>[12x]MPIVVTQAHIDRVGIAADLLDASPVSLQVLGRPTAINTV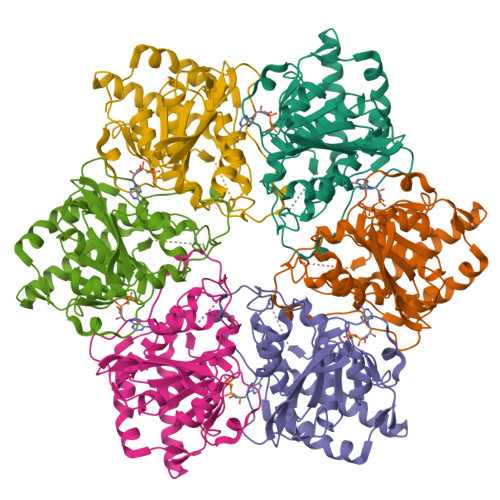VIKTYIAAVMELASKQGGSLAGVDIRPSVLLKDTAIFTKPKAKSADVESDVDVLDTGIYSVPGLARKPVTHRWPSEGIYSGVTALMGATGSGKSITLNEKLRPDVLIRWGEVAEAYDELDTAVHISTLDEMLIVCIGLGALGFNVAVDSVRPLLFRLKGAASAGGIVAVFYSLLTDISNLFTQYDCSVVMVVNPMVDAEKIEYVFGQVMASTVGAILCADGNVSRTMFRTNKGRIFNGAAPLAADTHMPSMDRPTSMKALDHTSIASVAP3-(4-phenylbutylamino)-1,4-bis(phenylmethyl)pyrrole-2,5-dione 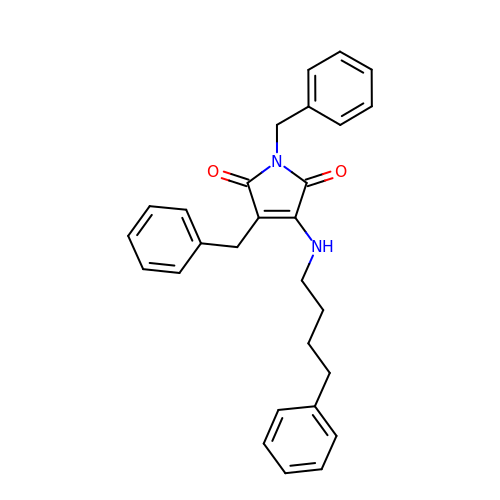| C28 H28 N2 O2 | QPFLANLQMKUFTC-UHFFFAOYSA-N>MIQEHRYDVVIVGAGGAGMRAAVEAGPRARTAVLTKLYPTRSHTGAAQGGMCAALANVEEDNWEWHTFDTVKGGDYLADQDAVEIMCKEAIDAVLDLEKMGMPFNRTPEGRIDQRRFGGHTRDHGKAPVRRACYAADRTGHMILQTLYQNCVKHDVEFFNEFYALDIALTETPAGPVATGVIAYELATGDIHVFHAKAIVFATGGSGRMYKTTSNAHTLTGDGLGIVFRKGLPLEDMEFHQFHPTGLAGLGILISEAVRGEGGRLLNGEGERFMERYAPTIVDLAPRDIVARSMVLEVLEGRGAGPNKDYVYIDVRHLGEDVLEAKLPDITEFARTYLGVDPVKELVPVYPTCHYVMGGIPTTVNGQVLRDNTNVIPGLYAAGECACVSVHGANRLGTNSLLDINVFGRRAGIAAAEYAQNHNFVDMPENPAEMVVGWVGDILSEHGNERVADIRGALQQSMDNNAAVFRTEETLKQALTDIHALKERYSRITVHDKGKRYNSDLLEAIELGFLLELAEVTVVGALNRKESRGGHAREDYPNRDDTNYMRHTMAYKQGTDLLSDIRLDYKPVVQTRYEPMERKY[3x];>MSAPVIDKPEAGDPELPPVPEGAVMVTLKIARFNPENPDAAGWQSFRVPCLPSDRLLNLLHYVKWYLDGTLTFRRSCAHGVCGSDAMRINGVNRLACKVLMRDMLPKNPNKQLTITIEPIRGLPVEKDLVVNMEPFFDAYRAVKPFLVTSGNPPTKERIQSPTDRARYDDTTKCILCACCTTSCPVYWSEGSYFGPAAIVNAHRFIFDSRDEAAAERLDILNEV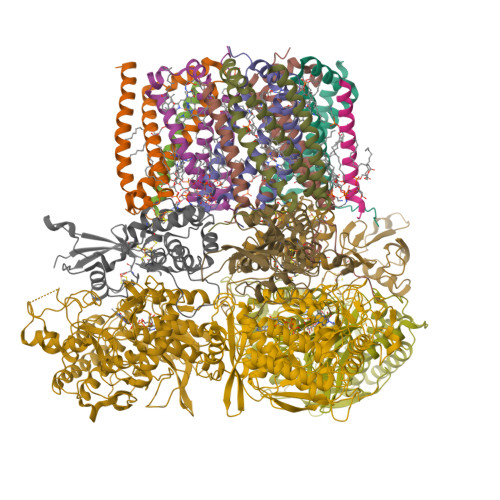DGVWRCRTTFNCTEACPRGIQVTQAIQEVKRALMFAR[3x];>MSTQTEVPAPQPKKTRRRTLYRGDPGMWSWVLHRITGATIFFFLFVHVLDTALVRVSPQAYNEVIETYKTPIVGLMEIGLVAAVLFHALNGIRVILIDFWAKGPRYQRQMLAVIAGLFLVIFIAAVGVIGMHMVERFL[3x];>[3x]MSAPGAGESRLGRPAPVMEREHDRPAALDHPRAPRKPRGIPYFEKYAWLFMRFSGIALVFLALGHLFIMLMWQDGVYRIDFNYVAERWASPFWQIWDMALLWLAMIHGANGMRTIIGDYARKNVTKFWLNSLLLLATGFTLVLGSYVLVTFDANISHHHHHHHHHH;>MVLFFEILLVAAVLVITWFAVYALYRLVTDES[3x]> MDIPRIFNITESAHRIHNPFTPEKLATLGAALRLEAGARV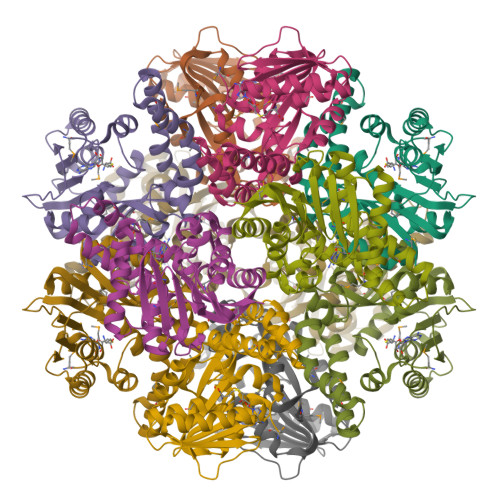LDLGSGSGEMLCTWARDHGIVGTGIDLSQLFTEQAKRRAEALGVAGQVKFIHGDAAGYVSDEKVDVAACVGASWIAGGVAGTITLLAQSLEPGGIILMGEPFWRKLPTTEAVAKACHANTISDFLLLPEFLASFRKLGYDVVEMVLADQDSWDRYEAAKWLTMRRWLDANPEDELAEEVRAQLSSEPERYATNTREYLGWGVFALMAR>[4x]SNAMSQFMNLEGKVALVTGASRGIGKAIAELLAERGAKVIGTATSESGAQAISDYLGDNGKGMALNVTNPESIEAVLKAITDEFGGVDILVNNAGITRDNLLMRMKEEEWSDIMETNLTSIFRLSKAVLRGMMKKRQGRIINVASVVGTMGNAGQANYAAAKAGVIGFTKSMAREVASRGVTVNTVAPGFIETDMTKALNDEQRTATLAQVPAGRLGDPREI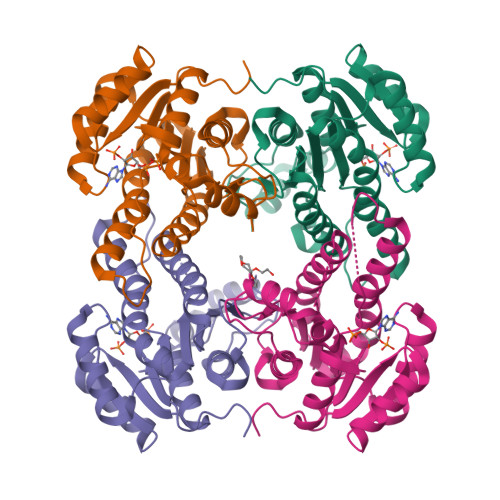ASAVAFLASPEAAYITGETLHVNGGMYMI> MERELPIPVFLTEDEDSVHERMLSNFQDVSTLEGDFIYDATRPTAEQIAELK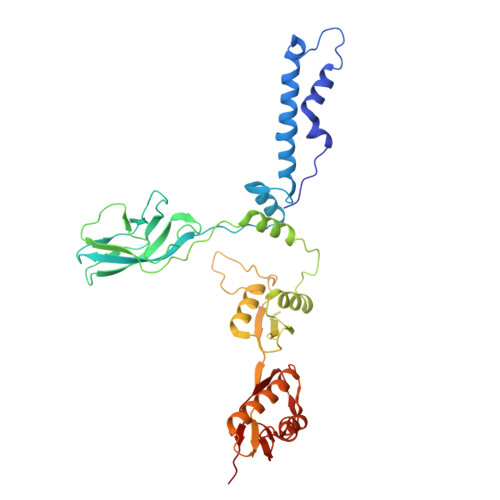QLGLQNNLKIAFPQTSYGTYLEWLGECKGVFKNQPTKATGVITFTGVQGTIITKGTIVTTIATDEKQSIEFELLETKTIGENETVDIKAESRIVGTIGNVSKGSISVLLGSISGVKSITNKEDFRGGTDIEDEEHFRERVLVAEQEDKLSGASSDYIRWAKEVDGVGYAYVVSEWAGAGTVKVLILDKNRKAATQELIDKVQEYIYPLNISEGENRDGKAPIGALVTVVTPDTLLINVKASFIFSNGFSEETVLNNLKTKIDKYLDKIDLGGTVSYNAIQAIVGSMMLTDEGIEDFSNLTINDVKENIKLQDQVVGIGEIVNEVVG>GHMSQTLKQLAMAKMAGFRHKTVVVPEWEGVKVVLREPSGEAWLRWQEVV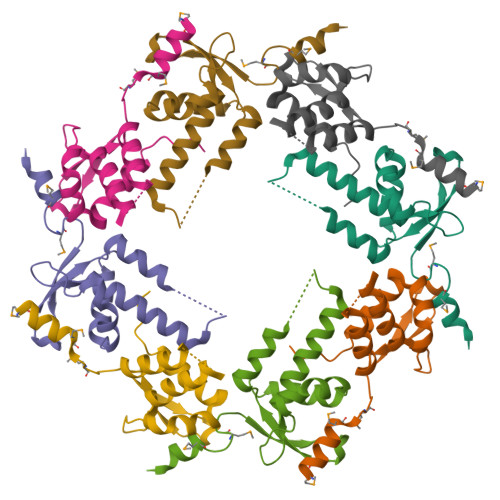KGGGDDENVSVSEKAHRNLCADVVLFIDVLCDTDKQPVFSVDEEEQVREIYGPVHSRLLKQALDLINNADEAREKSQPPA[2x]> MALLLASAINHTAHPAGLRSHPNNESFSRHHLCSSPQNISKRRSNLSFRPRAQTISSESAGIHRLSPWEIPRRDWFPPSFLFGAATSAYQIEGAWNEDGKGPSTWDHFCHNFPEWIVDRSNGDVAADSYHMYAEDVRLLKEMGMDAYRFSISWPRILPKGTLAGGINEKGVEYYNKLIDLLLENGIEPYITIFHWDTPQALVEAYGGFLDERIIKDYTDFAKVCFEKFGKTVKNWLTFNDPETFCSVSYGTGVLAPGRCSPGVSCAVPTGNSLSEPYIVAHNLLRAHAETVDIYNKYHKGADGRI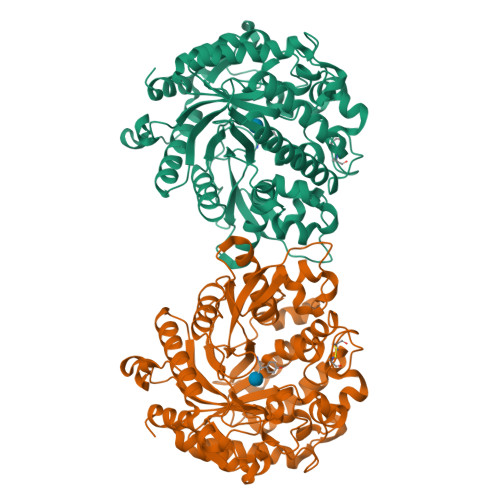GLALNVFGRVPYTNTFLDQQAQERSMDKCLGWFLEPVVRGDYPFSMRVSARDRVPYFKEKEQEKLVGSYDMIGINYYTSTFSKHIDLSPNNSPVLNTDDAYASQETKGPDGNAIGPPTGNAWINMYPKGLHDILMTMKNKYGNPPMYITENGMGDIDKGDLPKPVALEDHTRLDYIQRHLSVLKQSIDLGADVRGYFAWSLLDNFEWSSGYTERFGIVYVDRENGCERTMKRSARWLQEFNGAAKKVENNKILTPAGQLN>[2x]GPLGSVKNFELPKKHMQLNDFVKRVQESGIVKDAVIIHRLFDALTFGHEKQIDPETFRDFYTCWKETEAEAQEVSLPALLMEHLDKNECVYKLSSSVKTNRGVGKIAMT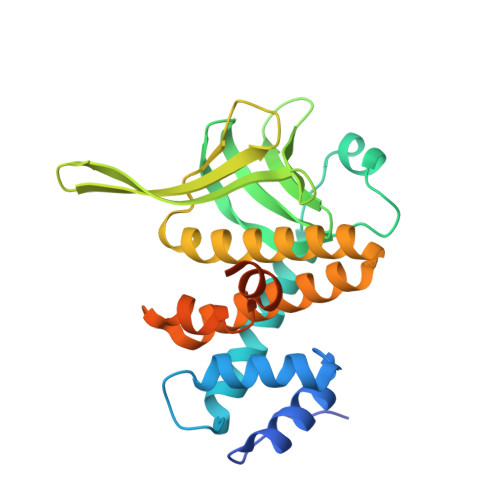QKRLFLLTEGRPGYVEIATFRNIEEVKNSTVAFLLLRIPTLKIKTVAKKEVFEANLKSECDLWHLMVKEMWAGKQLADDHKDPQYVQQALTNVLLMDAVVGTLQSPSAIHAASKLAYFDNMKKKSPMAVPKTTSETLKHKINPSAGETAP>[2x]MDYKFPKDFMFGTSTASYQIEGGWNEDGKGENIWDRLVHTSPEVIKDGTNGDIACDSYHKYKEDVAIIKDLNLKFYRFSISWARIAPSGVMNSLEPKGIAYYNNLINELIKNDIIPLVTMYHWDLPQYLQDLGGWVNPIMSDYFKEYARVLFTYFGDRVKWWITFNEPIAVCKGYSIKAYAPNLNLKTTGHY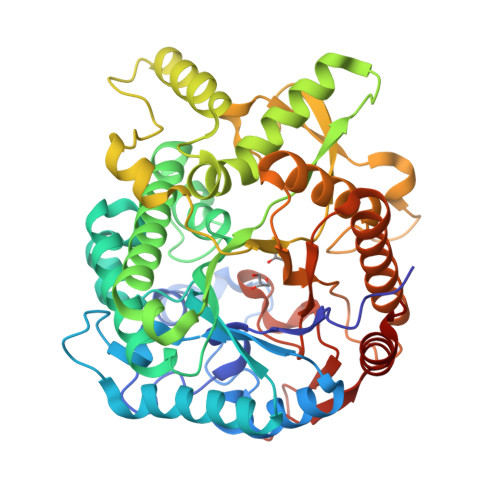LAGHTQLIAHGKAYRLYEEMFKPTQNGKISISISGVFFMPKNAESDDDIETAERANQFERGWFGHPVYKGDYPPIMKKWVDQKSKEEGLPWSKLPKFTKDEIKLLKGTADFYALNHYSSRLVTFGSDPNPNFNPDASYVTSVDEAWLKPNETPYIIPVPEGLRKLLIWLKNEYGNPQLLITENGYGDDGQLDDFEKISYLKNYLNATLQAMYEDKCNVIGYTVWSLLDNFEWFYGYSIHFGLVKIDFNDPQRTRTKRESYTYFKNVVSTGKP>AFTACEKQTIGKIAQVLAKSPEAYGAECLARLFVTHPGSKSYFEYKDYSAAGAKVQVHGGKVIRAVVKAAEHVDDLHSHLETLALTHGKKLLVDPQNFPMLSECIIVTLATHLTEFSPDTHCAVDKLLSAICQELSSRYR[2x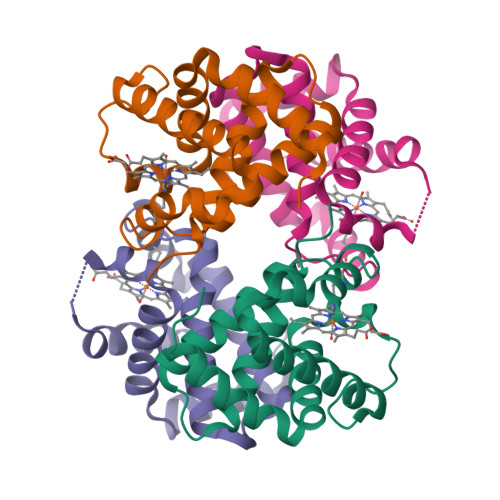];>VHWTQEERDEISKTFQGTDMKTVVTQALDRMFKVYPWTNRYFQKRTDFRSSIHAGIVVGALQDAVKHMDDVKTLFKDLSKKHADDLHVDPGSFHLLTDCIIVELAYLRKDCFTPHIQGIWDKFFEVVIDAISKQY[2x]> MDPTPVSVSGGTIHFEGKLVNAACAVSTKSADQTVTLGQYRTASFTAIGDTTAQVPFSIVLNDCDPKVAATAAVAFSGQADNTNTNLLAVSSADNSTTATGVGIEILDNTSSPLKPDGATFSAKQALVEGTNTLRFTARYKATAAATTPGQANADATFIMKYE;> MADPTPVSVSGGTIHFEGKLVNAACAVSTKSADQTVTLGQYRTASFTAIGDTTAQVPFSIVLNDCDPKVAATAAVAFSGQADNTNTNLLAVSSADNSTTATGVGIEILDNTSSPLKPDGATFSAKQALVEGTNTLRFTARYKATAAATTPGQANADATFIMKYE

The FimA subunits of the pilus rod are single domain proteins of 16 kDa with an incomplete, immunoglobulin (IG)2-like fold that lacks the C-terminal β-strand (G-strand). In the structure of the pilus rod, the FimA subunits interact via inter-molecular donor strand complementation, in which the N-terminal extension of each subunit, termed the donor strand, inserts as a β-strand into the preceding subunit and completes its IG-like fold. In 2010, Sukumaran et al. discovered that the FimA proteins from the enteroinvasive pathogens E. coli, Shigella flexneri, and Salmonella enterica have a second function besides formation of homopolymeric pilus rods; soluble forms of FimA, independent of FimC, act as inhibitors of host cell apoptosis after pathogen internalization by stabilizing the interaction between hexokinase and the voltage-dependent anion channel (VDAC) on the surface of mitochondria. We showed that all three FimA orthologues investigated (FimAECO, FimASHI, and FimASAL) were capable of folding to an alternative, self-complemented, monomeric form of only marginal thermodynamic stability that likely represents the FimA species that acts as an inhibitor of host cell apoptosis after internalization of the respective pathogen.

FimAECO, FimASHI, and FimASAL were produced as reduced, insoluble proteins in the E. coli cytoplasm without their N-terminal signal sequences. All proteins were refolded in the absence of the chaperone FimC under oxidizing conditions to allow the formation of the single, invariant structural disulfide bond. The purified proteins were crystallized, and their X-ray structures were determined at 1.5, 0.89, and 1.69 Å resolution, respectively. All FimA orthologues crystallized as self-complemented monomers, and all structures strongly resembled the previously reported NMR structure of the FimAECO monomer. Specifically, all three FimA monomers showed nearly identical immunoglobulin-like folds, completed by intramolecular donor strand insertion in a parallel orientation relative to the C-terminal F-strand. The global folds and registers of parallel donor strand insertion in the X-ray structures of FimASHI and FimASAL were the same as those observed in FimAECO, and all three structures showed high surface complementarity between donor strand and the rest of the folded FimA domain. The only significant difference in the mode of donor strand insertion was found for FimASAL, where Ser6 instead of Val5 occupied the P5 pocket, which caused a more extended conformation of the FimASAL donor strand segment Ser6–Gly7–Gly8. The overall pairwise Cα RMSD values for the three X-ray structures were 0.30 Å for FimAECO/FimASHI (113 Cα atoms), 0.51 Å for FimAECO/FimASAL (154 Cα atoms), and 0.57 Å for FimASAL/FimASHI (110 Cα atoms), and the only minor conformational differences were restricted to loop segments 15–20, 37–45, and 89–97, and residues 51 and 81.>GMSVIKPDMKIKLRMEGAVNGHPFAIEGVGLGKPFEGKQSMDLKVKEGGPLPFAYDILTMAFCYCYGNRVFAKYPENIVDYFKQSFPEGYSWERSMIYEDGGICNATNDITLDGDCYICEIRFDGVNFPANGPVMQKRTVKWELSTEKLYVRDGVLKSDGNYALSLEGGGHYRCDFKTTYKAKKVVQLPDYHSVDHHIEIISHDKDYSNVNLHEHAEA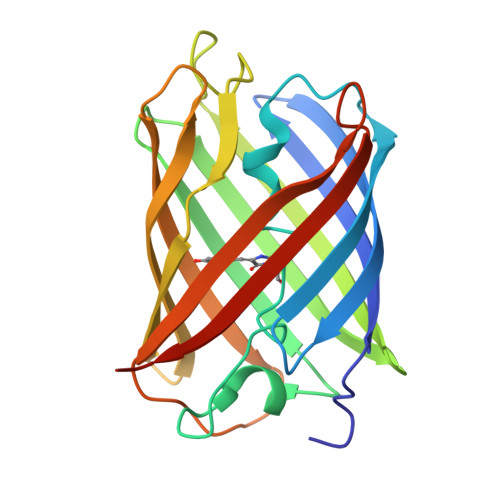HSELPRQAK[8x]>[2x]QIVTDNSIGNHDGYDYEFWKDSGGSGTMILNHGGTFSAQWNNVNNILFRKGKKFNETQTHQQVGNMSINYGANFQPNGNAYLCVYGWT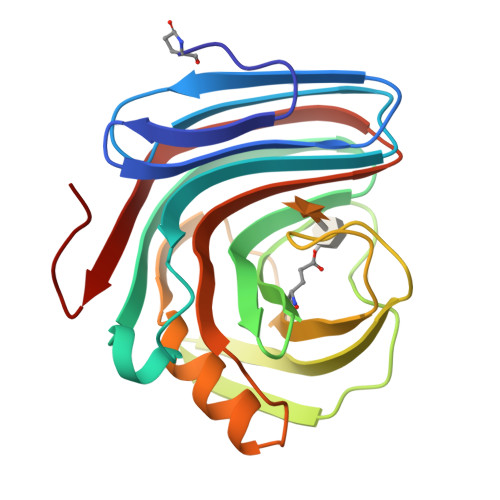VDPLVEYYIVDSWGNWRPPGATPKGTITVDGGTYDIYETLRVNQPSIKGIATFKQYWSVRRSKRTSGTISVSNHFRAWENLGMNMGKMYEVALTVEGYQSSGSANVYSNTLRINGNPLS> SNATGERFHPL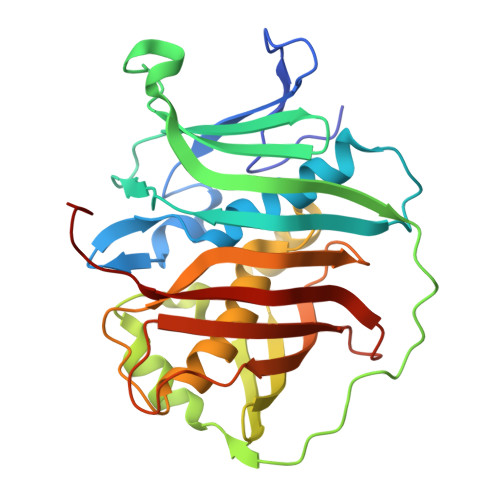LGRRVLDPAPGARCFTGTVSSDRPAYLGEHWVYDAIVVPGVTYLEMALAAASRLLPGNAADTLIVEDVTVWSPLVLRAGAPARLRLRSEDERFEIHSAEPERSDDESAWTRHATGRIARRQLSPDATGQLPRLDGEAVELDAYYERMRIYYGPRLRNIRHLERRGREAIGHVCLQGEEAQESASYELHPALLDACFQCVFALIYAHESHREPFVPLGCARIELRARGVREVRVHLRLHPPRSTDHNQTHTADLRLFDMEGRLVASVDALQLKRASKAALL(3S,6S)-N~3~-cyclopropyl-N~1~-(cyclopropylmethyl)-3,6-dimethylpiperazine-1,3-dicarboxamide | C15 H26 N4 O2 | 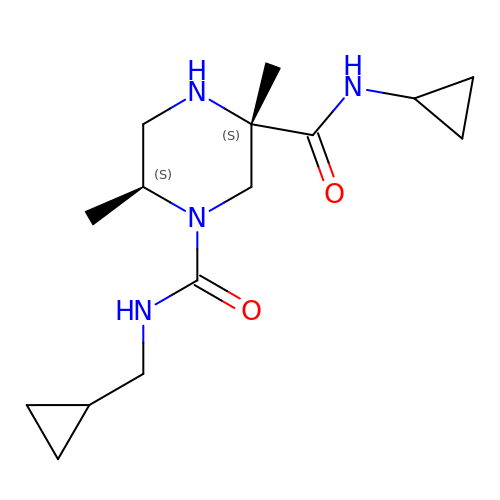SXNUQDJHCXDWNX-BONVTDFDSA-N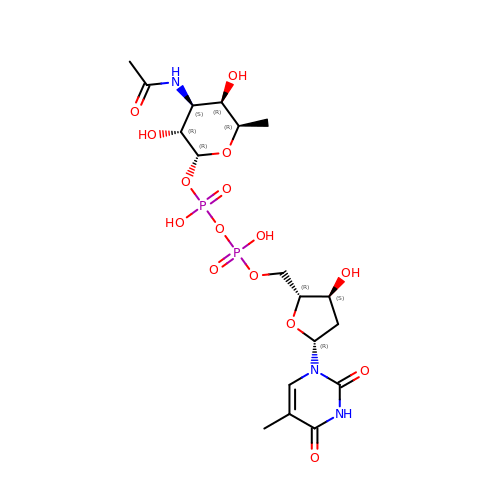[(2~{R},3~{R},4~{S},5~{R},6~{R})-4-acetamido-6-methyl-3,5-bis(oxidanyl)oxan-2-yl] [[(2~{R},3~{S},5~{R})-5-[5-methyl-2,4-bis(oxidanylidene)pyrimidin-1-yl]-3-oxidanyl-oxolan-2-yl]methoxy-oxidanyl-phosphoryl] hydrogen phosphate | C18 H29 N3 O15 P2 | CWQDRZJUANNJKC-HYPDDMKDSA-N>[10x]MQTTVTTMLLASVALAACAGGGSTPLPLPQQQPPQQEPPPPPVPLASRAACEALKDGNGDMVWPNAATVVEVAAWRDAAPATASAAALPEHCEVSGAIAKRTGIDGYPYEIKFRLRMPAEWNGRFFMEGGSGTNGSLSAATGSIGGGQIASALSRNFATIATDGGHDNAVNDNPDALGTVAFGLDPQAR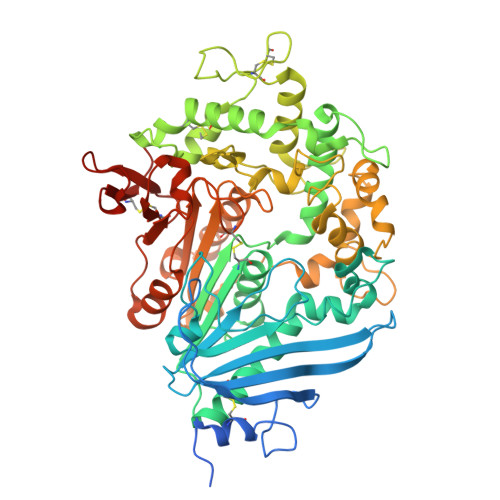LDMGYNSYDQVTQAGKAAVARFYGRAADKSYFIGCSEGGREGMMLSQRFPSHYDGIVAGAPGYQLPKAGISGAWTTQSLAPAAVGLDAQGVPLINKSFSDADLHLLSQAILGTCDALDGLADGIVDNYRACQAAFDPATAANPANGQALQCVGAKTADCLSPVQVTAIKRAMAGPVNSAGTPLYNRWAWDAGMSGLSGTTYNQGWRSWWLGSFNSSANNAQRVSGFSARSWLVDFATPPEPMPMTQVAARMMKFDFDIDPLKIWATSGQFTQSSMDWHGATSTDLAAFRDRGGKMILYHGMSDAAFSALDTADYYERLGAAMPGAAGFARLFLVPGMNHCSGGPGTDRFDMLTPLVAWVERGEAPDQISAWSGTPGYFGVAARTRPLCPYPQIARYKGSGDINTEANFACAAPPLEHHHHHH> FIFLALLGAAVAFPVDDDDKIVGGYTCGANTVPYQVSLNSGYHFCGGSLINSQWVVSAAHC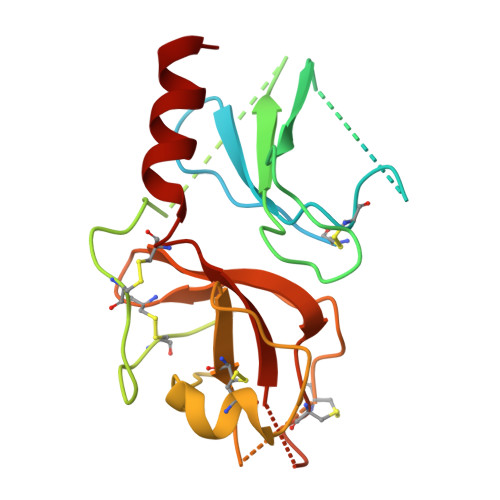YKSGIQVRLGEDNINVVEGNEQFISASKSIVHPSYNSNTLNNDIMLIKLKSAASLNSRVASISLPTSCASAGTQCLISGWGNTKSSGTSYPDVLKCLKAPILSDSSCKSAYPGQITSNMFCAGYLEGGKDSCQGDSGGPVVCSGKLQGIVSWGSGCAQKNKPGVYTKVCNYVSWIKQTIASN>[3x]GPAMKKLKPAPFYFQPFSKKQLKVLTWWRKASPVSDKDGIICDGSIRAGKTIVMSFSYVMWAMDTFNEQNFGMAGKTIGALRRNVITPLKRMLKSRGYRVKDHRADNYLTITFKGKTNYFYLFGGKDESSQDLIQGITLAGMFFDEVALMPESFVNQATARCSVDGAKLWFNCNPAGPYHWFKVEYLDKLDEKNLLHLHFTMDDNLSLSKQVKERYQRMYKGVFYQRYILGLWVLAEGIIYDMFDQDEHVVPTVPRPYEKYYVSCDYGTQNPTTFGLWGLYNGVWYKVKEYHYDGRKENKQKTDQEYYEDLMKFIEDIEKHKFKGVIVDPSAASFIALLRQKGIKVIKAKNDVLDGIRNVATALNKKMILYNDCCKETFREYSSYVWDEKAAERGEDKPVKQNDHQLDADRYFVNTILFGNKLRAVPSLY

Most dsDNA bacteriophages and viruses utilize a powerful DNA translocation motor to package their unit-length genome into a preformed procapsid. A central component of the motor, large terminase, consists of an N-terminal adenosine triphosphatase (ATPase) domain comprising ASCE (Additional Strand Catalytic glutamate) and lid subdomains, and a C-terminal nuclease domain, connected by a short linker sequence. While both domains are involved in interaction with DNA DNA translocation is powered by the ASCE subdomain using energy released coinciding with ATP hydrolysis. The nuclease domain is responsible for cleavage of the genomic DNA concatemer at both the initiation and completion stages of viral DNA packaging.

Subsequent soaking of these crystals in cryo-protectant containing a high concentration of NaCl resulted in a transition from R32 to C2 crystal form (Crystal form 2) with each of the ATPase domains of the three subunits related by the crystallographic 3-fold axis adopting a unique stable position. In the resulting C2 crystal form, there are three molecules in the asymmetric unit, each having a slightly different domain orientation, with an overall inter-subunit Cα rmsd of 0.8–1.6 Å. In this structure, the N-terminal ATPase and the C-terminal nuclease domains, tethered by a linker, adopt vastly different relative orientations to those observed in large terminases from other bacteriophages. In common with other phages, the N-terminal ATPase domain of the D6E terminase comprises both an ASCE and lid subdomains facing each other. From the lid subdomain, the polypeptide chain leads, through an ordered linker comprising 12 amino acids (230–241), into the C-terminal nuclease domain. The nuclease domain resembles the RNase H-like fold which, as found for the large terminases of other viruses, differs from other RNase H family proteins by an extended β-sheet and the presence of an auxiliary β-hairpin. Interestingly, the β-hairpin, previously predicted to interact with DNA, has an extended hairpin-like loop structure with an α-helix at its tip. The relative position of the ATPase and nuclease domains is stabilized by a salt bridge formed between R224 of the lid subdomain and D394 of the hairpin-like loop, and an interdomain hydrogen bond (M216-N362). There are also additional ATPase-nuclease domain–domain interactions resulting in a total surface area buried between the two domains of 362 Å2. For comparison, areas buried in inter-domain interactions in T4 and Sf6, are significantly smaller, 212 and 78 Å2, respectively. It is possible the distinct domain arrangement of the D6E large terminase stabilized by these interactions represents a biologically important conformationally locked inactive ‘initiation’ state that serves to prevent futile hydrolysis of ATP before assembly of this extremophilic motor.> MGNKICQFKLVLLGESAVGKSSLVLRFVKGQFHEFQESTIGAAFLTQTVCLDDTTVKFEIWDTAGQERYHSLA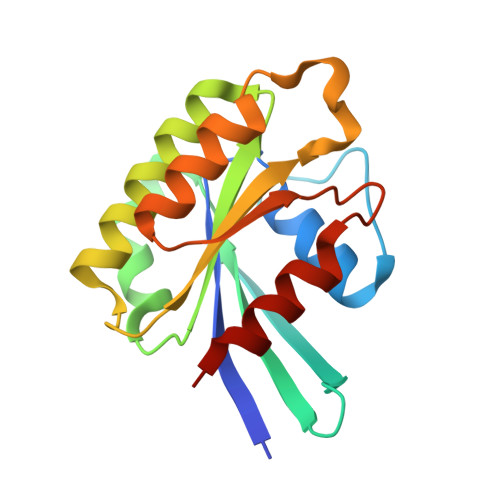PMYYRGAQAAIVVYDITNEESFARAKNWVKELQRQASPNIVIALSGNKADLANKRAVDFQEAQSYADDNSLLFMETSAKTSMNVNEIFMAIAKKLPKN>ADYIEMKVPAQPEYVGIIRLTLSGVASRMGYTYDEIEDLKIAVSEACTNAVQHAYKEDKNGEVSIRFGVFEDRLEVIVADEGDSFDFDQKQQDLGPYTPSHTVDQLSEGGLGLYLMETLMDEVRVQNHSGVTVAMTKYLNG[2x];>NINVDVKQNENDIQVNIAGEIDVYSAPVLREKLVPLAEQGADLRICLKDVSYMDSTGLGVFVGTFKMVKKQGGSLKLENLSERL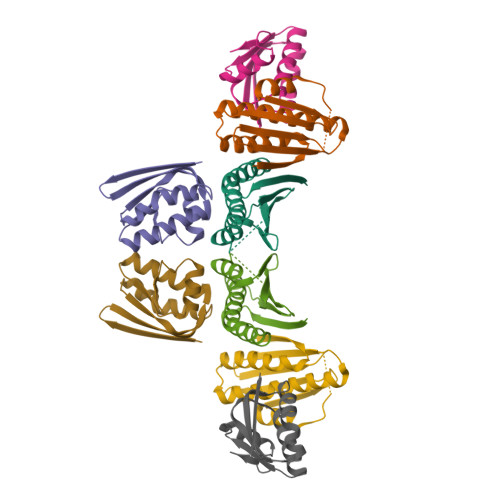IRLFDITGLKDIIDISAKS[2x]>[3x]GSDSIIHIGAIFDESAKKDDEVFRTAVGDLNQNEEILQTEKITFSVTFVDGNNPFQAVQEACELMNQGILALVSSIGCTSAGSLQSLADAMHIPHLFIQRSTAGTPRSGCGLTRSNRNDDYTLSVRPPVYLNEVILRVVTEYAWQKFIIFYDSEYDIRGIQEFLDKVSQQGMDVALQKVENNINKMITTLFDTMRIEELNRYRDTLRRAILVMNPATAKSFISEVVETNLVAFDCHWIIINEEINDVDVQELVRRSIGRLTIIRQTFPVPQNISQRCFRGNHRISSTLCDPKDPFAQNMEISNLYIYDTVLLLANAFHKKLQDRKWHSMASLSCIRKNSKPWQGGRSMLETIKKGGVNG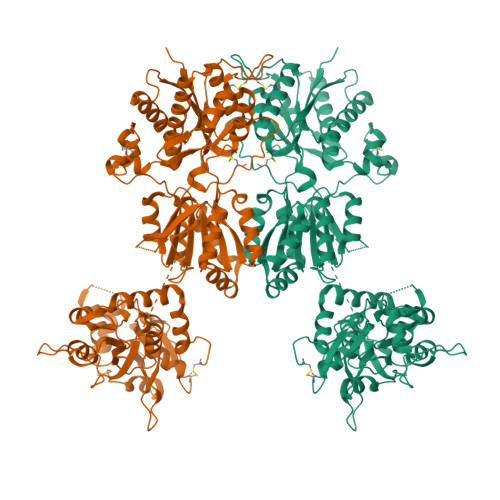LTGDLEFGENGGNPNVHFEILGTNYGEELGRGVRKLGCWNPVTGLNGSLTDKKLENNMRGVVLRVVTVLEEPFVMVSENVLGKPKKYQGFSIDVLDALSNYLGFNYEIYVAPDHKYGSPQEDGTWNGLVGELVFKRADIGISALTITPDRENVVDFTTRYMDYSVGVLLRRGTSIQSLQDLSKQTDIPYGTVLDSAVYQHVRMKGLNPFERDSMYSQMWRMINRSNGSENNVLESQAGIQKVKYGNYAFVWDAAVLEYVAINDPDCSFYTVGNTVADRGYGIALQHGSPYRDVFSQRILELQQSGDMDILKHKWWPKNGQCDLHHHHHH> MAPVPEPEVVATPPADAGRGLIRVDSREIRHYSGTRKEPDYLVSRDNGKTWEMKAAPAGYPPNYGGIPKESPAIVRNPLTREFIRVQPIGGFVFLSRGGLDGKWLAVTNDGKLEEDWKDPEKRKNLKKLGGIMRTPVFVNKGRRVIVPFHNMGGGTKFHISDDGGLTWHVSRNGVTSPRHEARPPHQGVRWFNNAVEATVLEMKDGTLWALARTSQDQAWQAFSKDYGETWSKPEPSRFFGTLTMNTLGRLDDGTIVSLWTNTMALPENATAGNGTWEDVFTNRDSHHIAMSGDEGKTWYGFREIILDEHRNHPGYATLDGPEDRGKHQSEMVQLDKNRILISLGQHKNHRRLVIVDRRWVGAKTRATQTGKDLDSQWTIHTYIPQKKGHCSYNRKPSAELVQDPSGGTKKVLQIKRLDDPELVNEKSNVDYRNGGATWNFPNGTTGLVKFRFRVVDGEQADDSGLQVSLTDRLFNACDSTTKDYALFTFPIRLKPAPHLLLGMKKVPFTPGAWHEISLLWQGGQAVVSLDGKKAGTLKMANKSPNGASYIHFISTGSQPDAGILLDTVNARVKAAAA;> MAPVPEPEVVATPPADAGRGLIRVDSREIRHYSGTRKEPDYLVSRDNGKTWEMKAAPAGYPPNYGGIPKESPAIVRNPLTREFIRVQPIGGFVFLSRGGLDGKWLAVTNDGKLEEDWKDPEKRKNLKKLGGIMRTPVFVNKGRRVIVPFHNMGGGTKFHISDDGGLTWHVSRNGVTSPRHEARPPHQGVRWFNNAVEATVLEMKDGTLWALARTSQDQAWQAFSKDYGETWSKPEPSRFFGTLTMNTLGRLDDGTIVSLWTNTMALPENATAGNGTWEDVFTNRDSHHIAMSGDEGKTWYGFREIILDEHRNHPGYATLDGPEDRGKHQSEMVQLDKNRILISLGQHKNHRRLVIVDRRWVGAKTRATQTGKDLDSQWTIHTYIPQKKGHCSYNRKPSAELVQDPSGGTKKVLQIKRLDDPELVNEKSNVDYRNGGATWNFPNGTTGLVKFRFRVVDGEQADDSGLQVSLTDRLFNACDSTTKDYALFTFPIRLKPAPHLLLGMKKVPFTPGAWHEISLLWQGGQAVVSLDGKKAGTLKMANKSPNGASYIHFISTGSQPDAGILLDTVNARVKAE

The mucolytic human gut microbiota specialist Akkermansia muciniphila is proposed to boost mucin-secretion by the host, thereby being a key player in mucus turnover. Mucin glycan utilization requires the removal of protective caps, notably fucose and sialic acid, but the enzymatic details of this process remain largely unknown. Here, we describe the specificities of ten A. muciniphila glycoside hydrolases, which collectively remove all known sialyl and fucosyl mucin caps including those on double-sulfated epitopes. Structural analyses revealed an unprecedented fucosidase modular arrangement and explained the sialyl T-antigen specificity of a sialidase of a previously unknown family.

To explain the strict specificity, we determined three structures of AmGH181: in ligand free form, bound with the transition-state inhibitor DANA (N-Acetyl-2,3-dehydro-2-deoxyneuraminic acid), and bound to both the T-antigen disaccharide (GNB) and DANA, which provides a mimic for a transition state-like substrate complex. At the catalytic site, R234 and R305 are shared with GH33, whereas glutamine (Q367) substitutes the third arginine in the GH33 conserved triad. A unique signature is the substitution of the tyrosine catalytic nucleophile in GH33 members to a glutamine (Q350) that is preceded by a histidine (H349) in AmGH181. Strikingly, Q350 and an adjacent glutamate (E218), both invariant in GH181, are potentially hydrogen bonded to a water molecule that overlays with the oxygen in the catalytic tyrosine of GH33 enzymes. This water is positioned for nucleophilic attack at the C2 of the sialyl (or the inhibitor) at subsite −1. Based on these data, we hypothesized that AmGH181 adopts an inverting mechanism that involves nucleophilic attack by the activated water molecule that overlays with the oxygen of the catalytic tyrosine in GH33 enzymes. The initial emerging signals were for β-Neu5Ac and α-Neu5Ac, in the reactions catalyzed by AmGH181 and AmGH33A, respectively. These data corroborated the proposed inverting mechanism of AmGH181, which is unprecedented in the evolutionary related CAZy clan E that includes GH33 retaining sialidases. The presence of two potential saccharide surface binding sites (SBSs) is intriguing. The first site is adjacent to the active site, where an inhibitor molecule was modelled, whereas a galactose unit was modelled at the second binding site located on the opposite side of the catalytic site.> MVASVSIQNVVKRYDKTTVVHGVSLDIEPGEFVVLVGPSGCGKSTTLRMVAGLEEISGGTIRIDGRVINDLAPKDRDVAMVFQNYALYPHLNVRDNISFGLRLKRTKKSVIDAAVKTAADILGLQPLLERKPSDLSGGQRQRVAMGRAIVRDPKVFLFDQPLSNLDAKLRTQMRAEIKRLHQRLGTTVIYVTHDQVEAMTLADRIVVMRDGLIEQIGKPMDLFLHPANTFVA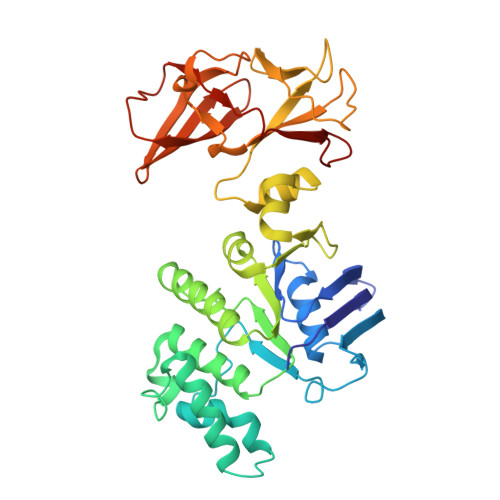SFIGSPPMNLMPARIAVDSTQHVELNGGNRISLLPRAGTHLAPGQEVVFGIRPEDVTLDGVEGSERAQIKATVDIVEPLGSESILHATVGDHSLVVKVGGLNEVHPGDPVTLHVDLTRVHLFDAQSQASIY> MEEKVESTTTPDGPCVVSVQETEKWMEEAMRMAKEALENIEVPVGCLMVYNNEVVGKGRNEVNQTKNATRHAEMVAIDQVLDWCHQHGQSPSTVFEHTVLYVTVEPCIMCAAALRLMKIPLVVYGCQNERFGGCGSVLNIASADLPNTGRPFQCIPGYRAEEAVELLKTFYKQENPNAPKSKVRKKDCQKS;> MEPTSGFAEQPGPVKAESEEQEPAQWQALPVLSEQQSGAVELILAYAAPVLDKRQTSRLLREVSAVYPLPAQPHLKRVRPSRSAGGAQSSDLLLCLAGPSAGPRSLAELLPRPAVDPRGLGTPFLVPVPARPPLTRSQFEEARAHWPTSFHEDKQVTSALAGQLFSTQERAAMQTHMERAVCAAQRAAAQGLRAVGAVVVDPASDRVLATGHDCSSVASPLLHAVMVCIDLVAQGQGEDSLPYV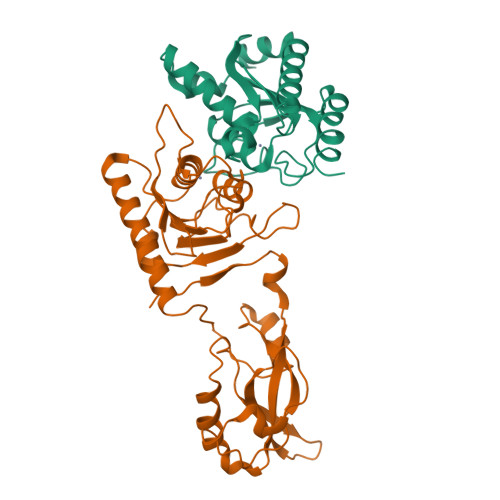CTGYDLYVTREPCVMCAMALVHARIQRVFYGAPSPDGALGTLFRVHARPDLNHRFQVFRGILEDQCRQLDPDP>MACPLEKALDVMVSTFHKYSGKEGDKFKLNKSELKELLTRELPSFLGKRTDEAAFQKLMSNLDSNRDNEVDF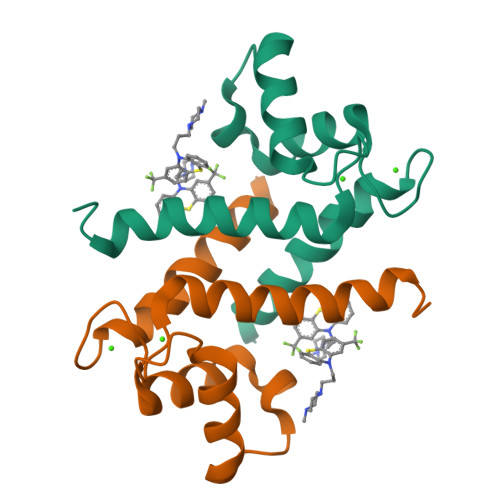QEYCVFLSCIAMMCNEFFEGFPDKQPRKK[20x]> GSHMSKKILIVESDTALSATLRSALEGRGFTVDETTDGKGSVEQIRRDRPDLVVLAVDLSAGQNGYLICGKL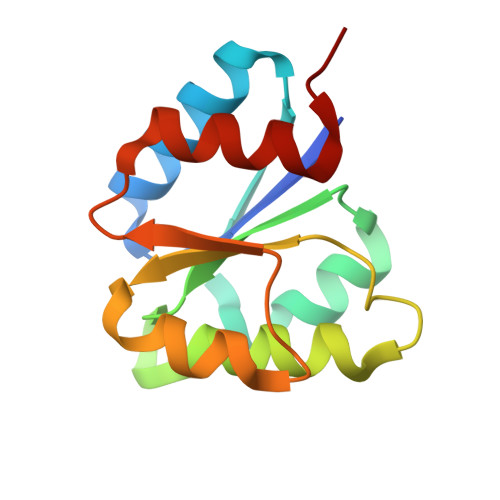KKDDDLKNVPIVIIGNPDGFAQHRKLKAHADEYVAKPVDADQLVERAGALIGFPE>[2x]MAHHHHHHVDDDDKMVHHDGFQTVKATIDWEHPMFKLYEKAKRNGKWNPADIDFSQDQKDFASLTSEEKISALPLVAGFSAGEEAVTLDILPMAHALARQGRLEDVLFLTTFMHDEAKH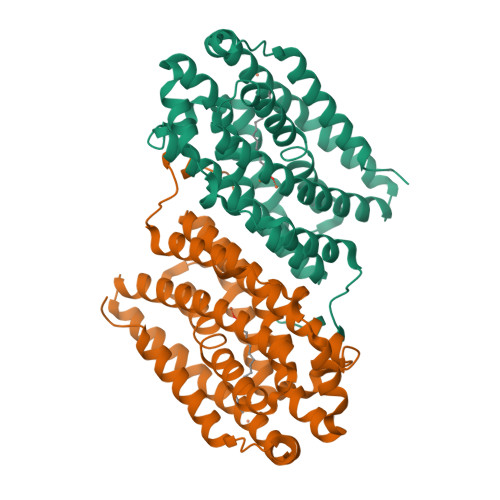VEMFSRWQQAVGIGQMDLSVFHNDHYKRIFYEALPEAMNRLYADDSPEAVIRAATVYNMIVEGTLAESGYYTFRQIYKKAGLFPGLLQGIDYLNMDEGRHIQFGIYTIQRIVNEDERYYELFIRYMDELWPHVIGYVDYLTELGKRQQQLARTYALEIDYDLLRHYVIKQFNLRKKQISRTKRVDVVEGLEKTAAES>GSFDLEDVRPNQTAKAEKATTSYQDEETKKKTKEELDKLMEPTLGVEAKIPRRNRALADKEGNRKATPDTTDELSEAQIMAIWNENIDEIPHLKELNDKTTSGLIYHSHDGKQEDKKRNLQYVRSGYVFDESYSEIVKNKNGVPYIFKNGIDGYIYYLGTSPSKELPKGNKVTYKGTWDFTSDVKTSYELSG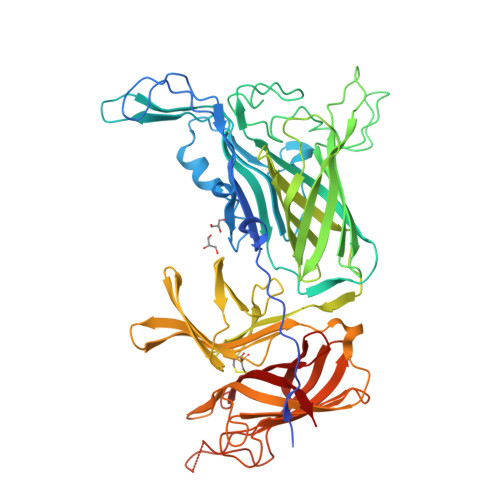FSDAGNGKNVAATSISDNVNRDHKVGEKLGDNEVKGVAHSSEFAVDFDNKKLTGSLYRNGYINRNKAQEVTKRYSIEADITGNRFRGKAKAEKAGDPIFTDSNYLEGGFYGPKAEEMAGKFFTNNKSLFAVFAAKSENGETTTERIIDATKIDLTQFNAKELNNFGDASVLIIDGQKIDLAGVNFKNSKTVEINGKTMVAVACCSNLEYMKFGQLWQKEGKQQVKDNSLFLQGERTATDKMPAGGNYKYVGTWDALVSKGTNWIAEADNNRESGYRTEFDVNFSDKKVNGKLFDKGGVNPVFTVDATINGNGFIGSAKTSDSGFALDAGSSQHGNAVFSDIKVNGGFYGPTAGELGGQFHHKSDNGSVGAVFGAKRQIEK[2x]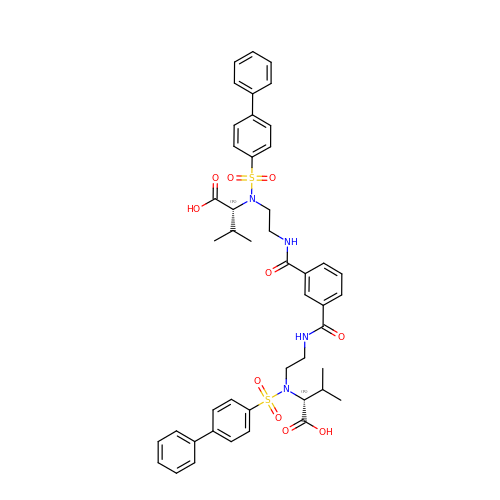N,N'-bis(2-[(biphenyl-4ylsulfonyl)[(2R)-1-hydroxy-3-methyl-1-oxobutan-2-yl]-amino]ethyl)benzene-1,3-dicarboxamide | C46 H50 N4 O10 S2 | JEFGHXXQQOIPKU-NCRNUEESSA-N> GPLGSDEILM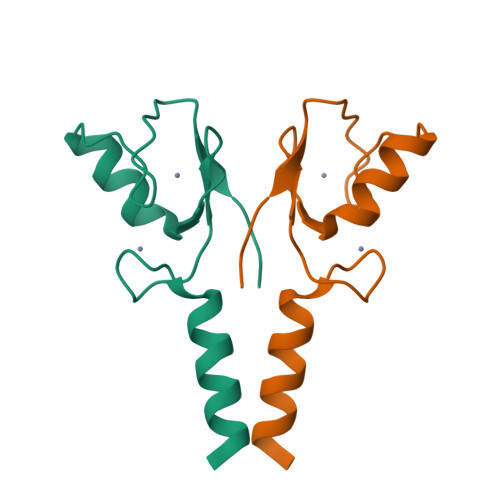EEIKDYKARLTCPCCNMRKKDAVLTKCFHVFCFECVKTRYDTRQRKCPKCNAAFGANDFHRIYIG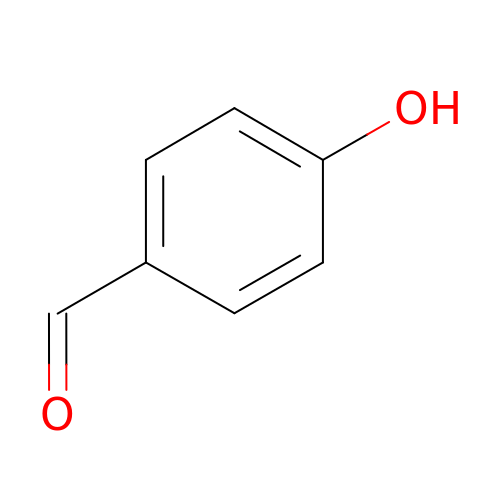P-HYDROXYBENZALDEHYDE | C7 H6 O2 | RGHHSNMVTDWUBI-UHFFFAOYSA-N> IVGGYTCEENSLPYQVSLNSGSHFCGGSLISEQWVVSAAHCYKTRIQVRLGEHNIKVLEGNEQFINAVKIIRHPKYNRDTLDNDIMLIKLSSPAVINARVSTISLPTAPPAAGTECLISGWGNTLSFGADYPDELKCLDAPVLTQAECKASYPGKITNSMFCVGFLEGGKDSCQRDSGGPVVCN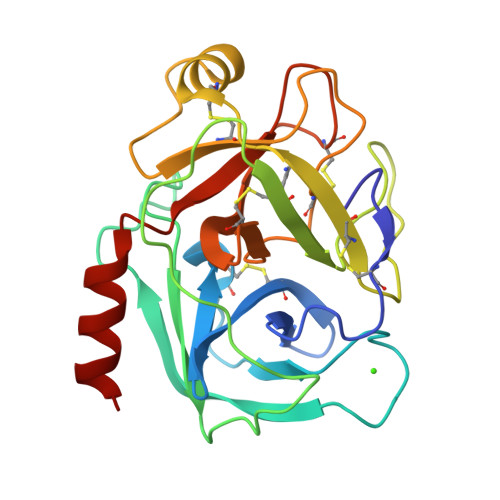GQLQGVVSWGHGCAWKNRPGVYTKVYNYVDWIKDTIAANS>[2x]MSKKRVVKLRELVPAVAALAVAVLIQSATGSSGGSGHTPTTQATHADDHDLTTHNGTEEHDDGHDDGHDDLHAHAPKVIVFISGSCLFGAISRSLFKKLPIPYTVVLLILGAILGVVASNVPLVEEHTRDVAHMDPHVLLQIFLPVL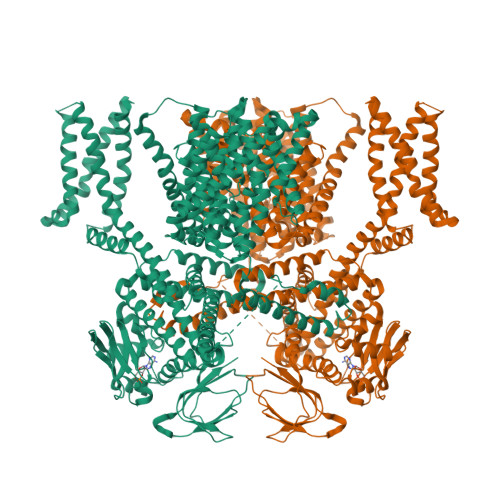IFESAFAMDVHTFMRSFSQVCILALFGLVVASVLTAVLAMNLFNYNWNFSEAMMFGAIMSATDPVAVVALLKDLGASKQLGTIIEGESLLNDGCAIVIFNVFMKMVFFPQLTSTVGQNVLYFLQVAVAGPLWGYAVAKVTVFFLSHIFNDALVEITITLAATYLTYYIGDIWLEVSGVLAVVVLGLIVNAEKTSISPEVEVFLHRFWEMLAYLANTLIFMMVGVVVTQKALVAVDKMDWFYLIILYLAITIIRGMVISLFSPILSRIGYGLTWRNAVIMTWGGLRGAVGLALALVVENLAGNDVIGSKFLFHTAGIVVLTLVINATTIQTLLRILGMSDISIPKRLAMAGAVRRIHEGQNRTLNMLKSDRFLADADWDIATAACEISDPYSALSDDENAPADELTLGERKSVCPGCKAMVPNEPSPREFADMMEEARLRMLKAEKISYWKQFEHGMLAREALRLLVQHAEVAADEKDQFILVDDLKKSWQIKGIYPWLKRKLEDLISEKKIAAIPMPKYKLGKLMYKICHHMAFEVTINIAIVLNIVPIIMEFVVQDKMASVSTMAAPGSTVSSEPSSLQKIEDALRISNYVFFVIYAIEAIVKILGLGRHYIVSHWNKFDAFILVVALVDIIIAETLLKGSITINLSSIKVVKLFRLLRGLRMLRLTKALIPKLILVVNGKINNQLSLGYDVGKGYIIGEEEVGKIIDRMVDNKKILRELKHISETGRLQVVKELGLLQREHPGIAVSVKTRQAIRTILNHSRETIHELQGAGLLDEMEAHKLELTVEIKMKRLMNAPSSIPPPPPENLLKNVSWLAGDMKLIDFIKARASLLHFDYGEVIVREGDESDGLFLIVSGLVKLYGKSAFLDHDNPPVTAGSEENEVFEDYLTVGNVIGEMGVLTKKPRNATVTCETTVQVYFITAEDMNIAIDTFTLYPSLEYRLWRVVAIRIATPLIMEQMAFQGWTQEKVKLHLERGYLVDLAESHFQFNIDATLEDVILINGTAYNAHTREEIRSPCLISRTVHKLTFQYTATEEPRLFVVRNAEYNGPILDGRLDVDSKRSLISITEISSNMCLKHAAELRQKNSKVMLSRKSSGAAAKEEEDCIPNTSDVEQAAGVSPSVPTKTTPKPKSFLPSLGLSMSKERVNGEAVEESPVKTKQGEETPETEEGAAPRVNVALEVLFQ> MKNIKKNQVMNLGPNSKLLKEYKSQLIELNIEQFEAGIGLILGDAYIRSRDEGKTYCMQFEWKNKAYMDHVCLLYDQWVLSPPHKKERVNHLGNLVITWGAQTFKHQAFNKLANLFIVNNKKTIPNNLVENYLTPMSLAYWFMDDGGKWDYNKNSTNTSIVLNTQSFTFEEVEYLVKGLRNKFQLNCYVKINKNKPIIYIDSMSYLIFYNLIKPYLIPQMM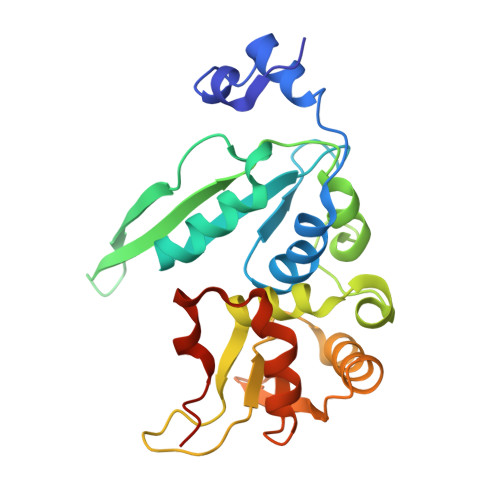YKLPNTISSETFLK>AAGTQGAEFPELCSYTWEAVDTKNNMLYKINICGNMGVAQCGPSSAVCMHDLKTDSFHSVGDSLLKTASRSLLEFNTTVNCKQQNHKIQSSITFLCGKTLGTPEFVTATDCVHYFEWRTTAACKKNIFKANKEVPCYAFDRELKKHDLNPLIKTSGAYLVDDSDPDTSLFINVCRDIEVLRASSPQVRVCPTGAAACLVRGDRAFDVGRPQEGLKLVSNDRLVLSYVKEGAGQPDFCDGHSPAVTITFVCPSERREGTIPKLTAKSNCRFEIEWVT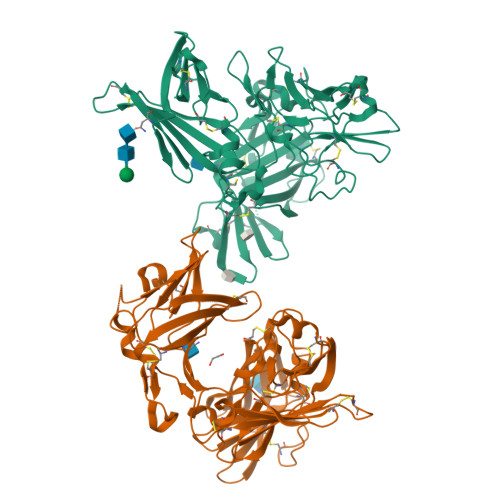EYACHRDYLESRSCSLSSAQHDVAVDLQPLSRVEASDSLFYTSEADEYTYYLSICGGSQAPICNKKDAAVCQVKKADSTQVKVAGRPQNLTLRYSDGDLTLIYFGGEECSSGFQRMSVINFECNQTAGNNGRGAPVFTGEVDCTYFFTWDTKYACV[2x]>MAHHHHHHMSTLLALDTSTEACSVALLHEGRALSHYEVIPRLHAQRLLPMVRDLLDEAGVALSAVDAIAFGRGPGAFTGVRIAIGVVQGLAFALQRPVLAVSDLAILAQRAYREQGAERVAAAIDARMDEVYWGCYQLQQGEMRLAGSEAVLPPERVAVPWDAAAADWFGAGTGWGYVERMPQRPVAL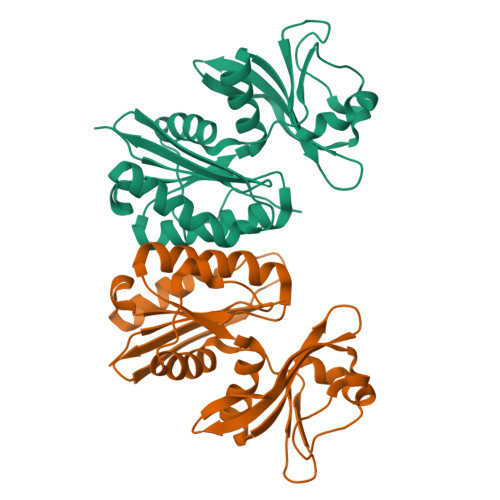DASLLPHAEDLLSLAGFAWARGEGVEAEQALPVYLRDNVATPKKAP[5x]>[2x]GPEKTDEYLLARFKGDGVKYKAKLIGIDDVPDARGDKMS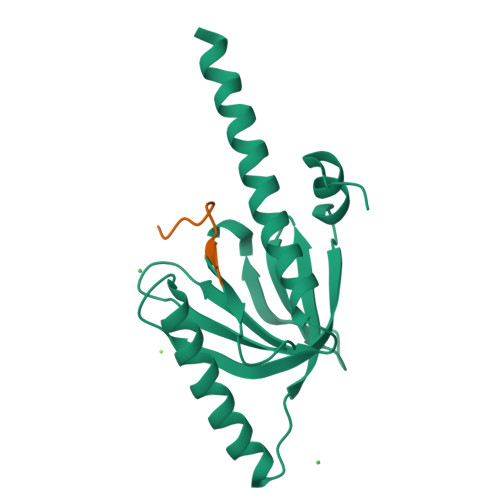QDSMMKLKGMAAAGRSQGQHKQRIWVNISLSGIKIIDEKTGVIEHEHPVNKISFIARDVTDNRAFGYVCGGEGQHQFFAIKTGQQAEPLVVDLKDLFQVIYNVKKKEEEKKKIEEASKAVEN;>XQNGFDNPNYQPQ[2x]> MTHQTHTIAESNNFIVLDKYIKAEPTGDSYQSESDLERELIQDLRNQGYEFISVKSQSAMLANVREQLQNLNGVVFNDSEWRRFTEQYLDNPSDGILDKTRKIHIDYICDFIFDDERLENIYLIDKKNLMRNKVQIIQQFEQAGSHANRYDVTILVNGLPLVQIELKKRGVAIREAFNQIHRYSKESFNSENSLFKYLQLFVISNGTDTRYFANTTKRDKNSFDFTMNWAKSDNTLIKDLKDFTATCFQKHTLLNVLVNYSVFDSSQTLLVMRPYQIAATERILWKIKSSFTAKNWSKPESGGYIWHTTGSGKTLTSFKAARLATELDFIDKVFFVVDRKDLDYQTMKEYQRFSPDSVNGSENTAGLKRNLDKDDNKIIVTTIQKLNNLMKAESDLPVYNQQVVFIFDECHRSQFGEAQKNLKKKFKRYYQFGFTGTPIFPENALGSETTASVFGRELHSYVITDAIRDEKVLKFKVDYNDVRPQFKSLETETDEKKLSAAENQQAFLHPMRIQEITQYILNNFRQKTHRTFPGSKGFNAMLAVSSVDAAKAYYATFKRLQEEAANKSATYKPLRIATIFSFAANEEQNAIGEISDETFDTSA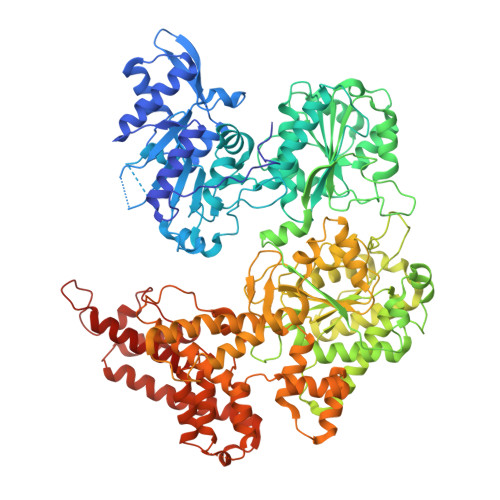MDSSAKEFLDAAIREYNSHFKTNFSTDSNGFQNYYRDLAQRVKNQDIDLLIVVGMFLTGFDAPTLNTLFVDKNLRYHGLMQAFSRTNRIYDATKTFGNIVTFRDLERSTIDAITLFGDKNTKNVVLEKSYTEYMEGFTDAATGEAKRGFMTVVSELEQRFPDPTSIESEKEKKDFVKLFGEYLRAENILQNYDEFATLKALQQIDLSDPVAVEKFKAEHYVDDEKFAELQTIRLPADRKIQDYRSAYNDIRDWQRREKEAEKKEKSTTDWDDVVFEVDLLKSQEINLDYILGLIFEHNRQNKGKGEMIEEVKRLIRSSLGNRAKEGLVVDFIQQTNLDDLPDKASIIDAFFTFAQREQQREAEALIKEENLNEDAAKRYIRTSLKREYATENGTELNETLPKLSPLNPQYKTKKQAVFQKIVSFIEKFKGVGGKI> LDLFVSPLGRVEGDLDVRVTINDGVVTSAWTEAAMFRGFEIILRGKDPQAGLIVCPRICGICGGSHLYKSAYALDTAWRTHMPPNATLIRNICQACETLQSIPRYFYALFAIDLTNKNYAKSKLYDEAVRRFAPYVGTSYQPGVVLSAKPVEVYAIFGGQWPHSSFMVPGGVMSAPTLSDVTRAIAILEHWNDNWLEKQWLGCSVDRWLENKTWNDVLAWVDENESQYNSDCGFFIRYCLDVGLDKYGQGVGNYLATGTYFEPSLYENPTIEGRNAALIGRSGVFADGRYFEFDQANVTEDVTHSFYEGNRPLHPFEGETIPVNPEDGRRQGKYSWAKSPRYAVPGLGNVPLETGPLARRM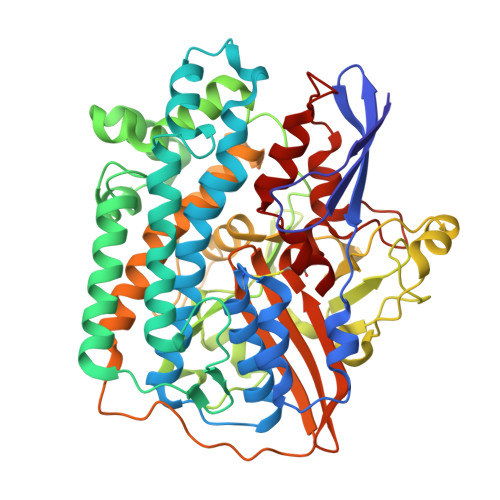AASAPDAETHQDDDPLFADIYNAIGPSVMVRQLARMHEGPKYYKWVRQWLDDLELKESFYTKPVEYAEGKGFGSTEAARGALSDWIVIEDSKIKNYQVVTPTAWNIGPRDASEVLGPIEQALVGSPIVDAEDPVELGHVARSFDSCLVCTVH> LG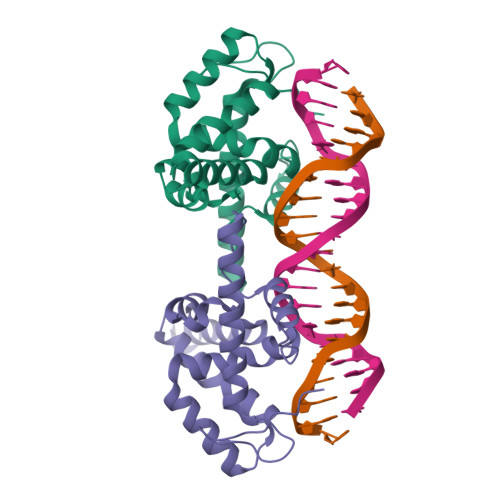TERQREHPFIVTEPGEVARGKKNGLDYLFHLYEQCREFLLQVQTIAKDRGEKCPTKVTNQVFRYAKKSGASYINKPKMRHYVHCYALHCLDEEASNALRRAFKERGENVGSWRQACYKPLVNIACRHGWDIDAVFNAHPRLSIWYVPTKLRQLCHLERNNAVAAAAALVGGISCTGSSTSGRGGCGGDDLRF>GSMAQILPIRFQEHLQLQNLGINPANIGFSTLTMESDKFICIREKVGEQAQVVIIDMNDPSNPIRRPISADSAIMNPASKVIALKAGKTLQIFNIEMKSKMKAHTMTDDVTFWKWISLNTVALVTDNAVYHWSMEGESQPVKMFDRHSSLAGCQIINYRTDAKQKWLLLTGISAQQNRVVGAMQLYSVDRKVSQPIEGHAASFAQFKMEGNAEESTLFCFAVRGQAGGKLHIIEVGTPPTGNQPFPKKAVDVFFPPEAQNDFPVAMQISEKHDVVFLITKYGYIHLYDLETGTCIYMNRISGETIFVTAPHEATAGIIGVNRKGQVLSVCVEEENIIPYITNVLQNPDLALRMAVRNNLAGAEEL[2x];>SDILFPADS[4x]

Clathrin mediates vesicular transport between post‐Golgi membranes in eukaryotes and is targeted to specific membranes by interactions with clathrin adaptor proteins. A total of 3 consensus clathrin‐binding peptide sequences have been identified and structural studies show that each binds distinct sites on the clathrin heavy chain N‐terminal domain (NTD). We have solved high‐resolution structures of NTD bound to peptide motifs from the cellular clathrin adaptors β2 adaptin and amphiphysin plus a putative viral clathrin adaptor, hepatitis D virus large antigen (HDAg‐L). Surprisingly, with each peptide we observe simultaneous peptide binding at multiple sites on NTD and viral peptides binding to the same sites as cellular peptides.

The viral peptides (HDAg‐L1pep and HDAg‐L2pep) bound at a similar site on NTD. However, in both cases only 2 consecutive hydrophobic side chains could be observed in the hydrophobic pocket (“IL” and “LL” in the cases of HDAg‐L1pep and HDAg‐L2pep, respectively). Interestingly, for both HDAg‐L1pep and HDAg‐L2pep the residues bound at the clathrin box do not match predictions based on alignments to the CBM consensus sequence, 18: in HDAg‐L1pep residues “ILFPA” occupy the positions corresponding to the LΦxΦ[DE], whereas in HDAg‐L2pep the residues “LLES”, including a C‐terminal serine residue that is non‐native and was added to the peptide to aid solubility, occupy the positions equivalent to the first 4 residues of the LΦxΦ[DE] consensus. There was not strong evidence for the HDAg‐L1pep peptide bound at the arrestin box. In addition to binding at the clathrin and arrestin boxes, in 3 of the NTD:peptide co‐crystal structures solved (Amph4T1pep, HDAg‐L1pep and HDAg‐L2pep) a bound peptide could be observed lying across the interface between blades 6 and 7 of the NTD β‐propeller. In the co‐structure with Amph4T1pep a phenylalanine side chain projects deep into this pocket while in the HDAg‐L1pep and HDAg‐L2pep structures the side chains of a leucine residue and proline residue, respectively, bind less deeply. In addition, in the co‐structures with HDAg‐L1pep and Amph4T1pep the backbone carbonyl oxygen of F9 forms a hydrogen bond with a backbone amide nitrogen of the bound peptide, and backbone atom(s) of E11 form hydrogen bond(s) with the bound peptide (1 bond in the case of HDAg‐L1pep, 2 in the case of Amph4T1pep). Despite the similar molecular interactions made between the Royle box and the bound peptides, we note that the direction of the peptide chain differs between HDAg‐L1pep and Amph4T1pep/HDAg‐L2pep. Previous cell‐based studies showed that mutation of HDAg‐L1 L199 to alanine severely reduced VLP production and clathrin co‐immunoprecipitation. This is consistent with our structure, as L199 forms extensive hydrophobic contacts at both the Royle and clathrin boxes.>[4x]MAHHHHHHVGTGSNDDDDKSPDPNWELVYTARLQMVKVLAVLYDGGEHAKQVPGLLGTTENELGLRKWLEDQGHTLVTTSDKDREGSTFDREL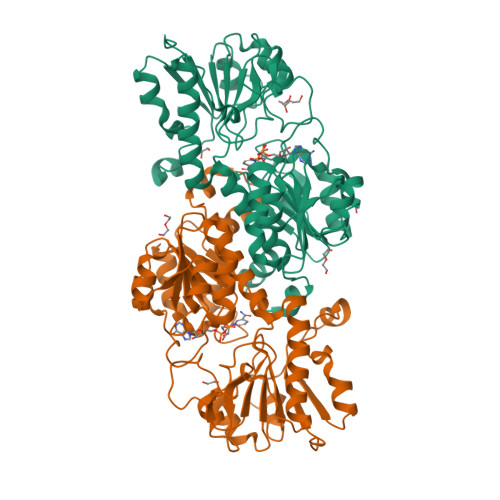EDAEIIITTPFHPGYLTAERLARAKKLKLAVTAGIGSDHVDLDAANKTNGGITVAEVTGSNVVSVAEHVVMTILVLVRNFVPAHEQIEAGRWDVAEVAKDEYDLEGKVVGTVGVGRIGERVLRRLKGFDCKELLYYDYQPLSPEKEKEIGCRRVENLEEMLAQCDVVTINCPLHESTRGLFNKDLISKMKRGSWLVNTARGAIVVKEDVAEALRTGHLRGYGGDVWFPQPAPADHVLRTAKNPFGGGNAMVPHMSGTSLDAQKRYAEGVKRILDSYLSGRFDYRPEDLIVHQGKYATRAYGQREDVKIPGQHHHHHH>ALGSMFGCLVAGRLVQTAAQQVAEDKFVFDLPDYESINHVVVFMLGTIPFPEGMGGSVYFSYPDSNGMPVWQLLGFVTNGKPSAIFKISGLKSGEGSQHPFGAMNIVRTPSVAQIGISVELLDSMAQQTPVGNAAVSSVDSFTQFTQKMLDNFYNFASSFAVSQAQMTPSPSEMFIPANVVLK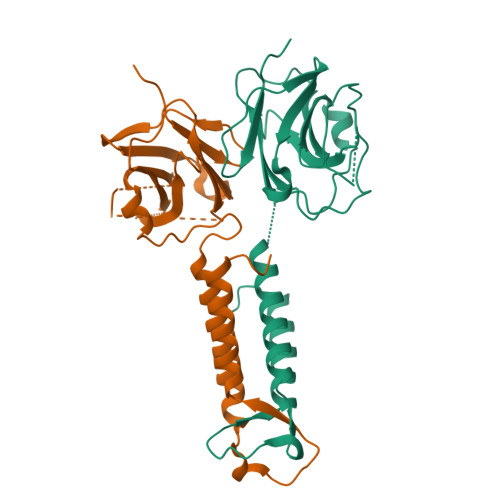WYENFQRRLAQNPLFWKT[2x]>[2x]DTIYKMNKSTRGIAVIINNKDFLRSSGMDRYPRNGTDVDRDALAKLFRALKFDVRIYNNQTRAEIRRITKEMAITNHTPY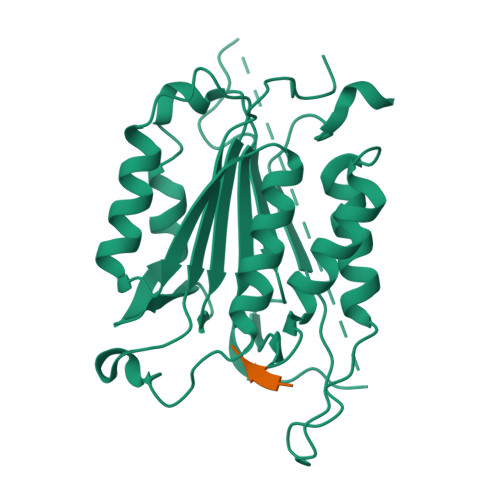DAFIFSILTHGEEGVIYGTDGTMAIKDLTAIFKDCTTLVGKPKMFFFQACQGHEYMDGVSVPAEADFVYAYSTVPGYYSWRNSVNGSWFIQSLTKVFEENAERMDILRMLTRVNAMVSTYKSRTGDYYSDSKRQVSSVVSMLRKELYFFPENV;> KLFSFGG;>XDEVD[2x]> KQVDVHDPVMTREGATWYLFSTGPGITIYSSKDRVNWRYSDRAFATEPTWAKRVSPSFDGHLWAPDIYQHKGLFYLYYSVSAFGKNTSAIGVTVNKTLNPASPDYRWEDKGIVIESVPQRDLWNAIAPAIIADDHGQVWMSFGSFWGGLKLFKLNDDL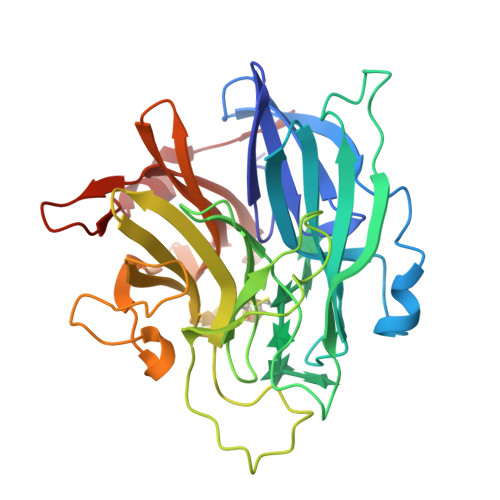TRPAEPQEWHSIAKLERSVLMDDSQAGSAQIEAPFILRKGDYYYLFASWGLCCRKGDSTYHLVVGRSKQVTGPYLDKTGRDMNQGGGSLLIKGNKRWVGLGHNSAYTWDGKDYLVLHAYEAADNYLQKLKILNLHWDGEGWPQVDEKELDSYISQRL> GSHMDFVAFMNKINSINANLSRYENIINQIDAQHKDLLTQVSEEQEMELRRSLDDYISQATDLQYQLKADIKDAQRDGLHDSNKQAQAENCRQKFLKLIQDYRIIDSNYKEESKEQAKRQYTIIQPEATDEEVEAAINDVNGQQIFSQALLNANRRGEAKTALAEVQARHQELLKLEKTMAELTQLFNDMEELVIE;>QGHMSNFLAEQYERDRKAIINCCFSRPDHKTGEPPNNYITHVRIIEDSKFPSSRPPPDSKLENKKKRLLILSAKPNNAKLIQIHKARENSDGSFQIGRTWQLTELVRVEKDLEISEGFILTMSKKYYWETNSAKERTVFIKSLITLYIQTFEGHVPELVNWDLSLFYLDERSYQRAVITNRPGSVSPIKSPTSNFTTNTTQSVGSVPFSAPTERTRRSETESVNPVSTPASVEYHAGMKSLNKAPYSSNS[2x]

The exocyst is an evolutionarily conserved octameric protein complex that mediates the tethering of post-Golgi secretory vesicles to the plasma membrane. Most syntaxin proteins contain an N-terminal region that autonomously folds into a three-helix bundle (the ‘Habc domain') that interacts intramolecularly with their SNARE motif to generate a ‘closed' conformation, which, in many cases, blocks its assembly into the SNARE complex345678910. The rate-limiting step is the interaction between Sso and Sec9, which is hindered by the auto-inhibition of Sso. Here we report that the exocyst subunit Sec3 directly interacts with Sso1/2, and promotes the initial assembly of the Sso-Sec9 t-SNARE complex and stimulates membrane fusion.

We have obtained the crystal structure of the Sec3–Sso2 complex under two different crystallization conditions, both of which demonstrate that the binding of Sec3 leads to conformational changes on Sso that is crucial for the relief of its auto-inhibition. The interface between Sec3N and Sso2 is ∼700 Å2, which is mediated primarily by 13 hydrogen bonds and 10 salt bridges. The seven main interface residues on Sec3 consist of K149, Q219, E222, H224, Y237, R241 and R245, which together describe a horseshoe-like shape on a relatively flat surface of the Sec3 PH domain. These residues provide a platform to make extensive contacts with Hc of Sso2, and some contacts with the SNARE motif of Sso2. Additionally, side chains of residues R241 and R245 of Sec3 form a finger-like structure that cradles around Hc and reach to the Ha motif of Sso2. In the Sso2-Sec3 crystal structure, the N terminus of the H3 domain bends approximately 22° away from its original position, and is tilted towards the Ha domain. The crystal structure suggests that Sec3 interaction causes the bending of the SNARE motif, which then led to the disruption of the hydrophobic interactions in the core of Sso2 involving HL2. The four Sec3/Sso2 dimers in the two crystal forms are essentially identical. Both the bending of the SNARE motif N-terminus and the relaxation of HL2 of Sso2 described above are found in all four copies of the Sec3/Sso2 complex present in the two different crystal forms.> MSLSFCGNNISSYNIYHGVLQNPCFVDALNLVPHVFLLFITFPILFIGWGSQSSKVQIHHNTWLHFPGHNLRWILTFALLFVHVCEIAEGIVSDSQRASRHLHLFMPAVMGFVATTTSIVYYHNIETSNFPKLLLALFLYWVMAFITKTIKLVKYWQLGWGMSDLRFCITGVMVILNGLLMAVEINVIRVRRYVFFMNPQKVKPPEDLQDLGVRFLQPFVNLLSKATYWWMNTLIISAHRKPIDLKAIGKLPIAMRAVTNYVCLKEAYEEQKKKAADHPNRTPSIWLAMYRAFGRPILLSSTFRYLADLLGFAGPLCISGIVQRVNEPKNNTTRFSETLSSKEFLENAHVLAVLLFLALILQRTFLQASYYVTIETGINLRGALLAMIYNKILRLSTSNLSMGEMTLGQINNLVAIETNQLMWFLFLCPNLWAMPVQIIMGVILLYNLLGSSALVGAAVIVLLAPIQYFIATKLAEAQKSTLDYSTERLKKTNEILKGIKLLKLYAWEHIFCKSVEETRMKELSSLKTFALYTSLSIFMNAAIPIAAVLATFVTHAYASGNNLKPAEAFASLSLFHILVTPLFLLSTVVRFAVKAIISVQKLNEFLLSDEIGEDSWRTGEGTLPFESCKKHTGVQSKPINRKQPGRYHLDNYEQARRLRPAETEDVAIKVTNGYFSWGSGLATLSNIDIRIPTGQLTMIVGQVGCGKSSLLLAILGEMQTLEGKVYWNNVNESEPSFEATRSRSRYSVAYAAQKPWLLNATVEENITFGSSFNRQRYKAVTDACSLQPDIDLLPFGDQTEIGERGINLSGGQRQRICVARALYQNTNIVFLDDPFSALDIHLSDHLMQEGILKFLQDDKRTVVLVTHKLQYLTHADWIIAMKDGSVLREGTLKDIQTKDVELYEHWKTLMNRQDQELEKDMEADQTTLERKTLRRAMYSREAKAQMEDEDEEEEEEEDEDDNMSTVMRLRTKMPWKTCWWYLTSGGFFLLFLMIFSKLLKHSVIVAIDYWLATWTSEYSINDPGKADQTFYVAGFSILCGAGIFLCLVTSLTVEWMGLTAAKNLHHNLLNKIILGPIRFFDTTPLGLILNRFSADTNIIDQHIPPTLESLTRSTLLCLSAIGMISYATPVFLIALAPLGVAFYFIQKYFRVASKDLQELDDSTQLPLLCHFSETAEGLTTIRAFRHETRFKQRMLELTDTNNIAYLFLSAANRWLEVRTDYLGACIVLTASIASISGSSNSGLVGLGLLYALTITNYLNWVVRNLADLEVQMGAVKKVNSFLTMESENYEGTMDPSQVPEHWPQEGEIKIHDLCVRYENNLKPVLKHVKAYIKPGQKVGICGRTGSGKSSLSLAFFRMVDIFDGKIVIDGIDISKLPLHTLRSRLSIILQDPILFSGSIRFNLDPECKCTDDRLWEALEIAQLKNMVKSLPGGLDATVTEGGENFSVGQRQLFCLARAFVRKSSILIMDEATASIDMATENILQKVVMTAFADRTVVTIAHRVHTILTADLVIVMKRGNILEYDTPESLLAQEDGVFASFVRADM

ATP-sensitive potassium channels (KATP), composed of Kir6 and SUR subunits, convert the metabolic status of the cell into electrical signals. Functional KATP channels are hetero-octamers composed of four Kir6 subunits and four SUR subunits. SUR subunits are not only targeted by inhibitors, such as insulin secretagogues, but also by activators, such as KATP openers. Here, we present cryo-EM structures of SUR2A and SUR2B subunits in complex with Mg-nucleotides and P1075 or levcromakalim, two chemically distinct KATP openers that are specific to SUR2.

We first solved the cryo-EM structure of SUR2B in the presence of Mg-ADP/Mg-ATP but without KATP openers to the resolution of 3.4 Å. The ABC transporter core of SUR2 shows an occluded state, which is similar to SUR1 in Mg-nucleotide-bound KATP structures. However, the density of TMD0 was missing due to its flexibility, suggesting that TMD0 was unstable without co-assembly with the Kir6 channel. For better visualization of the position of Lev, a fragment of TMD2 in front of Lev was omitted in (b); the residual detergent densities are also omitted. d Empty KATP opener-binding site in the cryo-EM map of the SUR2B subunit in complex with Mg-nucleotides is outlined by dashed lines. We observed that Mg-nucleotides are bound to both nucleotide-binding sites of SUR2. Although we prepared the SUR2B + P1075 samples using Mg-ATP alone, while other SUR2 samples using both Mg-ADP and Mg-ATP, we found that Mg-ATP was bound in the degenerate site and Mg-ADP was bound in the consensus site in all of the structures. As a result, ATP is tightly sandwiched between NBD1 and NBD2, and the degenerate site is fully closed. However, as the C-loop of the opposing NBD1 is away from Mg-ADP, the consensus site is still open. Upon binding of Mg-ADP to NBD2 of SUR2, NBD1 and NBD2 dimerize asymmetrically, with the degenerate site fully closed while the consensus site remains open. The dimerization of NBDs further drives the closure of TMD1 and TMD2 and the occlusion of TMD.>[2x]SMSSAIKSYKSVLRPNERKNQLLKSTIQCLEDGSAFFFKMLQGLFGGITPEIVRFSTEQEKQQQDIALWCAVNWFRPVSQDSLTHTIASDNLVEKFEEYYGGTASDAIKQYFSASIGESYYWNDCRQQYYDLCRELGVEVSDLTHDLEILCREKCLAVATESNQNNSIISVLFGTGEKEDRSVKLRITKKILEAISNLKEIPKNVAPIQEIILNVAKATKETFRQVYAGNLGAPSTLEKFIAKDGQKEFDLKKLQTDLKKVIRGKSKERDWCCQEELRSYVEQNTIQYDLWAWGEMFNKAHTALKIKSTRNYNFAKQRLEQFKEIQSLNN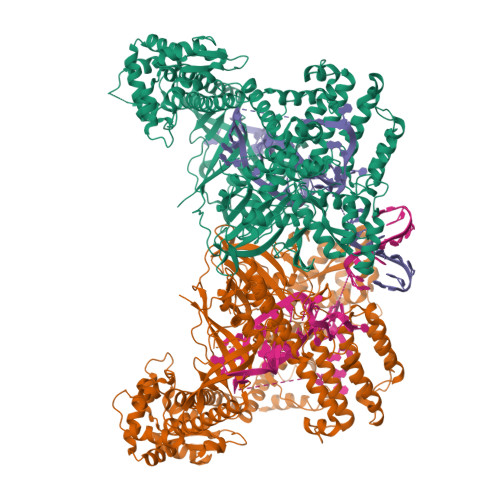LLVVKKLNDFFDSEFFSGEETYTICVHHLGGKDLSKLYKAWEDDPADPENAIVVLCDDLKNNFKKEPIRNILRYIFTIRQECSAQDILAAAKYNQQLDRYKSQKANPSVLGNQGFTWTNAVILPEKAQRNDRPNSLDLRIWLYLKLRHPDGRWKKHHIPFYDTRFFQEIYAAGNSPVDTCQFRTPRFGYHLPKLTDQTAIRVNKKHVKAAKTEARIRLAIQQGTLPVSNLKITEISATINSKGQVRIPVKFDVGRQKGTLQIGDRFCGYDQNQTASHAYSLWEVVKEGQYHKELGCFVRFISSGDIVSITENRGNQFDQLSYEGLAYPQYADWRKKASKFVSLWQITKKNKKKEIVTVEAKEKFDAICKYQPRLYKFNKEYAYLLRDIVRGKSLVELQQIRQEIFRFIEQDCGVTRLGSLSLSTLETVKAVKGIIYSYFSTALNASKNNPISDEQRKEFDPELFALLEKLELIRTRKKKQKVERIANSLIQTCLENNIKFIRGEGDLSTTNNATKKKANSRSMDWLARGVFNKIRQLAPMHNITLFGCGSLYTSHQDPLVHRNPDKAMKCRWAAIPVKDIGDWVLRKLSQNLRAKNIGTGEYYHQGVKEFLSHYELQDLEEELLKWRSDRKSNIPCWVLQNRLAEKLGNKEAVVYIPVRGGRIYFATHKVATGAVSIVFDQKQVWVCNADHVAAANIALTVKGIGEQSSDEENPDGSRIKLQLTS> AHHHHHHHRSDAAVIVVGAGPAGMMLAGELRLAGVEVVVLE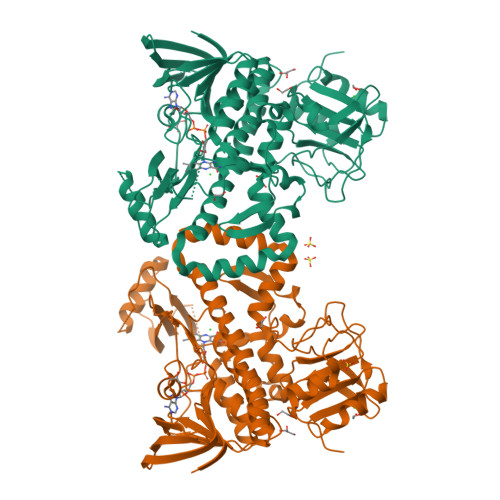RLVERTGESRGLGFTARTMEVFDQRGILPRFGEVETSTQGHFGGLQFDFGVLEGAWQAAKTVPQSVTETHLEQWATGLGADIRRGHEVLSLTDDGAGVTVEVRGPEGKHTLRAAYLVGCDGGRSSVRKAAGFDFPGTAATMEMYLADIKGVELQPRMIGETLPGGMVMVGPLPGGITRIIVCERGTPPQRRETPPSWHEVADAWKRLTGDDIAHAEPVWVSAFGNATRQVTEYRRGRVILAGDSAHIHLPAGGQGMNTSIQDAVNLGWKLGAVVNGTATEELLDSYHSERHAVGKRLLMNTQAQGLLFLSGPEVQPLRDVLTELIQYGEVARHLAGMVSGLEITYDVGTGSHPLLGKRMPALELTTATRETSSTELLHTARGVLLDLADNPRLRARAAAWSDRVDIVTAVPGEVSATSGLRDTTAVLIRPDGHVAWAAPGSHHDLPMALERWFGAPLTG> GPNVCAVQKVIGTNRKYFTNCKQWYQRKICGKSTVISYECCPGYEKVPGEKGCPAALPLSNLYETLGVVGSTTTQLYTDRTEKLRPEMEGPGSFTIFAPSNEAWASLPAEVLDSLVSNVNIELLNALRYHMVGRRVLTDELKHGMTLTSMYQNSNIQIHHYPNGIVTVNCARLLKADHHATNGVVHLIDKVISTITNNIQQIIEIEDTFETLRAAVAASGLNTMLEGNGQYTLLAPTNEAFEKIPSETLNRILGDPEALRDLLNNHILKSAMCAEAIVAGLSVETLEGTTLEVGCSGDMLTINGKAIISNKDILATNGVIHYIDELLIPDSAKTLFELAAESDVSTAIDLFRQAGLGNHLSGSERLTLLAPLNSVFKDGTPPIDAHTRNLLRNHIIKDQLASKYLYHGQTLETLGGKKLRVFVYRNSLCIENSCIAAHDKRGRYGTLFTMDRVLTPPMGTVMDVLKGDNRFSMLVAAIQSAGLTETLNREGVYTVFAPTNEA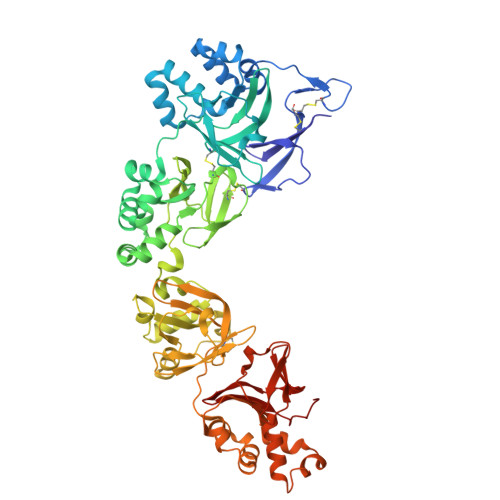FRALPPREWSRLLGDAKELANILKYHIGDEILVSGGIGALVRLKSLQGDKLEVSLKNNVVSVNKEPVAEPDIMATNGVVHVITNVLHHHHHH>SNAASLVHQPHPLEHSWTFWFDNPSAKSKQATWGASIRPIYTFSTVEEFWSVYNNIHHPSKLAMRADLYCFKHKIEPKWEDPVCANGGKWTVNFPRGKSDNGWLYTLLAMIGEQFDCGDEICGAVVNVRSGQDKISIWTKNASNEAAQASIGKQWKEFL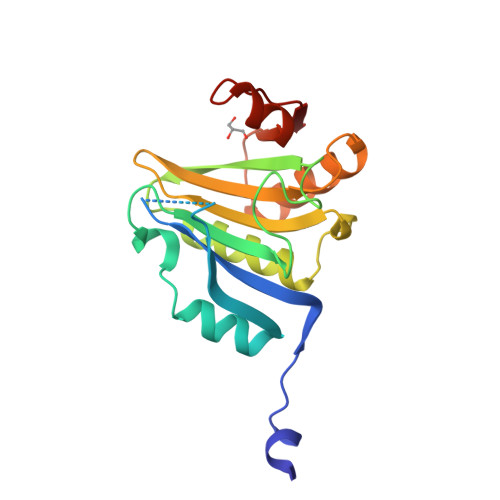DYNESIGFIFHDDAKKFDRHAKNKYMV[4x]>MELWLVRHGETLWNREGRMLGWTDLPLTAEGEAQARRLKGALPSLPAFSSDLLRARRTAELAGFSPRLYPELREIHFGALEGALWETLDPRYKEALLRFQGFHPPGGESLSAFQERVFRFLEGLKAPAVLF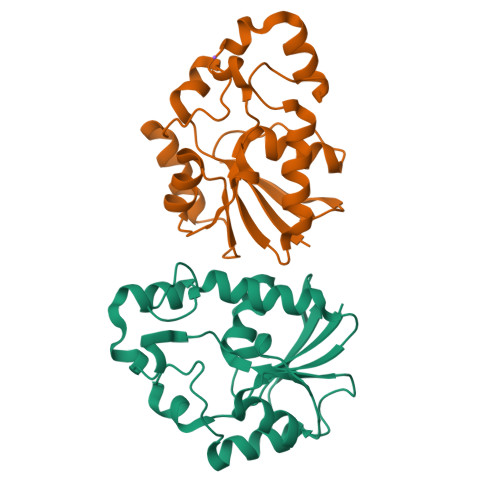THGGVVRAVLRALGEDGLVPPGSAVAVDWPRRVLVRLALDGEEATG[2x]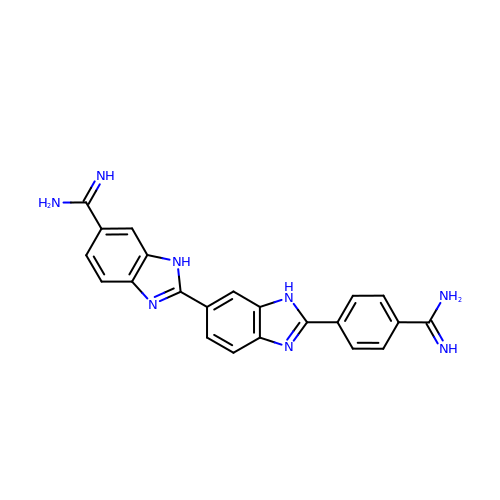5-AMIDINO-2-[2-(4-AMIDINOPHENYL)-5-BENZIMIDAZOLYL]BENZIMIDAZOLE | C22 H18 N8 | YEJMAZMIHIFTFO-UHFFFAOYSA-N> GSMAAAGNKSINAK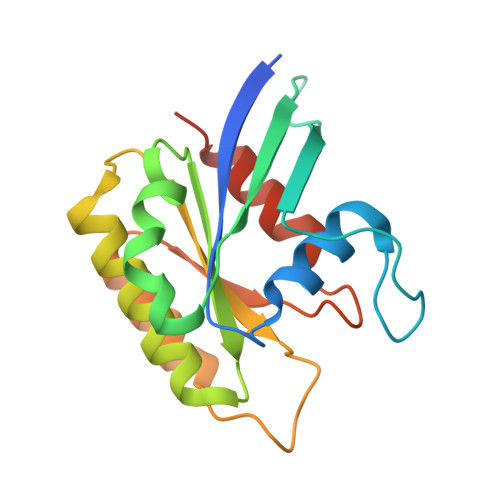LVLLGDVGAGKSSLVLRFVKDQFVEFQESTIGAAFFSQTLAVNDATVKFEIWDTAGQERYHSLAPMYYRGAAAAIIVFDVTNQASFERAKKWVQELQAQGNPNMVMALAGNKSDLLDARKVTAEDAQTYAQENGLFFMETSAKTATNVKEIFYEIARRLPRVQPTEN> GPLGSASLFATITGASKTEWSFSDIELTYRPNTLLSLGVMEFTLPSGFTANTKDTMNGNALRTTQILNNGKTVRVPLALDLLGAGEFKLKLNNKTL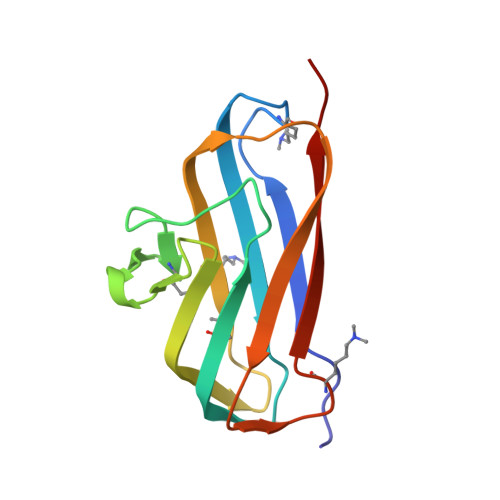PAAGTYTFRAENKSLSIGNKFYAEASIDVAKRST> GSAKDPLIKLKNFTELNS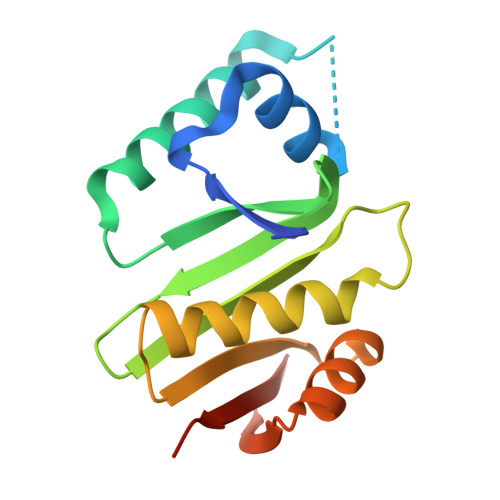QEIELIFKWRNHPDINQFMKTKYIDFEEHLRFLKKLHQDSSKKYFLVFQDEQIIGVIDFVNITTKSCEFGLYAKPNLKGVGQILMNEIIKYAFESLKVNTLKAYVFKSNHKALKLYQQNHFTIYDEDKDFYYVYLKQSNCKALPS The capsaicin- and heat-activated receptor, TRPV1, has served as a model for deciphering lipid modulation, which is relevant to understanding how pro-algesic agents enhance channel activity in the setting of inflammatory pain. Identification of a pocket within the TRPV1 transmembrane core has provided initial clues as to how phosphoinositide lipids bind to and regulate the channel. Here we show that this regulatory pocket in rat TRPV1 can accommodate diverse lipid species, including the inflammatory lipid lysophosphatidic acid, whose actions are determined by their specific modes of binding. We captured several states of TRPV1 ranging from channels in which the VBP is empty to those bearing different bioactive lipids, including distinct phosphoinositide species, brominated phosphoinositide analogs and a pro-algesic lipid, lysophosphatidic acid (LPA). Together, our data show how the VBP accommodates a range of bioactive lipids and how occupancy of the site corresponds to the structural status of the pore.

To resolve this question, we exploited our ability to generate TRPV1 protein with an empty vanilloid pocket, into which we introduced tetrabrominated analogs of PI or PIP2 (PI–Br4 and PIP2–Br4, respectively) as contrast-enhancing probes to distinguish these lipids from the other, unbrominated lipids in the nanodiscs. Previous work has established that brominated lipids are faithful analogs of the unsaturated lipids from which they are synthesized. In these high-resolution structures (2.2–2.4 Å resolution), we were able to identify the bromine atoms within the oleoyl tails of the lipids by visually comparing the resulting reconstructions against those previously determined for samples containing endogenous lipids. The well-resolved inositol headgroup of the bound lipids showed the expected differential location of phosphate moieties, most notably at the 4 and 5 positions for PIP2. Furthermore, conformations of both PI- and PIP2-reconstituted channels resemble the apo channel containing a native resident lipid. Together, these data demonstrate that the vanilloid site can accommodate PI or PIP2, where they act as negative regulatory factors to stabilize the closed state.

>[2x]MEQRASLDSEESESPPQENSCLDPPDRDPNCKPPPVKPHIFTTRSRTRLFGKGDSEEASPLDCPYEEGGLASCPIITVSSVLTIQRPGDGPASVRPSSQDSVSAGEKPPRLYDRRSIFDAVAQSNCQELESLLPFLQRSKKRLTDSEFKDPETGKTCLLKAMLNLHNGQNDTIALLLDVARKTDSLKQFVNASYTDSYYKGQTALHIAIERRNMTLVTLLVENGADVQAAANGDFFKKTKGRPGFYFGELPLSLAACTNQLAIVKFLLQNSWQPADISARDSVGNTVLHALVEVADNTVDNTKFVTSMYNEILILGAKLHPTLKLEEITNRKGLTPLALAASSGKIGVLAYILQREIHEPECRHLSRKFTEWAYGPVHSSLYDLSCIDTCEKNSVLEVIAYSSSETPNRHDMLLVEPLNRLLQDKWDRFVKRIFYFNFFVYCLYMIIFTAAAYYRPVEGLPPYKLKNTVGDYFRVTGEILSVSGGVYFFFRGIQYFLQRRPSLKSLFVDSYSEILFFVQSLFMLVSVVLYFSQRKEYVASMVFSLAMGWTNMLYYTRGFQQMGIYAVMIEKMILRDLCRFMFVYLVFLFGFSTAVVTLIEDGKYNSLYSTCLELFKFTIGMGDLEFTENYDFKAVFIILLLAYVILTYILLLNMLIALMGETVNKIAQESKNIWKLQRAITILDTEKSFLKCMRKAFRSGKLLQVGFTPDGKDDYRWCFRVDEVNWTTWNTNVGIINEDPGNCEGVKRTLSFSLRSGRVSGRNWKNFALVPLLRDASTRDRHATQQEEVQLKHYTGSLKPEDAEVFKDSMVPGEK Potassium channels propagate electrical signals, maintain membrane potentials and facilitate numerous downstream cellular processes. KirBac3.1 adopts the canonical fold of a K+ channel, with inner and outer membrane-spanning helices supporting an inclined, shorter, pore helix that supports the signature selectivity filter. All feature an hourglass-like constriction at the intracellular opening, leading to the widespread conclusion that the canonical permeation gate at the helix bundle crossing is closed (or nearly so) in all Kir structures, whether determined by crystallography or single-particle cryo-EM. Thus, data presented here indicate that inward rectifiers (Kir) are able to conduct without requiring the substantial conformational changes predicted by the canonical gating mechanism.

A near atomic resolution crystal structure (2.0 Å) of wild-type KirBac3.1 was determined, providing an accurate starting model for simulations. Steered molecular dynamics simulations, in which K+ ions are moved from the transmembrane cavity to the cytosol, were carried out on the pore of KirBac3.1 (residues 33–138 of the 2.0 Å structure) embedded in a POPC membrane separating saline reservoirs. Over the duration of the simulations the narrowness of the shallow intracellular opening did not prevent K+ passing through. The simulations report free-energy barriers at the Tyr132 collar of 6 kJ mol−1 for wild type and 1 kJ mol−1 for the disulfide-linked mutant. These values fall within the range expected for thermal fluctuations and are too low to impair K+ flux. Within the pore cavity, K+ diffuses with a coordination number of approximately six. A fleeting reduction in the number of solvating water molecules to three or four occurs as the ion passes through the collar of tyrosine side chains but is almost immediately replenished. Transient interactions between K+ and the Tyr132-hydroxyl groups occur after the ions pass the low energetic barrier near the center of the tyrosine aromatic ring. The retention of a kernel of water molecules means the free-energy barrier to permeation at the constriction is not prohibitive.

> MTGGMKPPARKPRILNSDGSSNITRLGLEKRGWLDDHYHDLLTVSWPVFITLITGLYLVTNALFALAYLACGDVIENARPGSFTDAFFFSVQTMATIGYGKLIPIGPLANTLVTLEALCGMLGLAVAASLIYARFTRPTAGVLFSSRMVISDFEGKPTLMMRLANLRIEQIIEADVHLVLVRSEISQEGMVFRRFHDLTLTRSRSPIFSLSWTVMHPIDHHSPIYGETDETLRNSHSEFLVLFTGHHEAFAQNVHARHAYSCDEIIWGGHFVDVFTTLPDGRRALDLGKFHEIAQHHHHHH> SKSKVDNQFYSVEVGDSTFTVLKRYQNLKPIGSGAQGIVCAAYDAVLDRNVAIKKLSRPFQNQTHAKRAYRELVLMKCVNHKNIISLLNVFTPQKTLEEFQDVYLVMELMDANLCQVIQMELDHERMSYLLYQMLCGIKHLHSAGIIHRDLKPSNIVVKSDCTLKILDFGLARTAGTSFMMTPYVVTRYYRAPEVILGMGYKENVDIWSVGCIMGEMVRHKILFPGRDYIDQWNKVIEQLGTPCPEFMKKLQPTVRNYVENR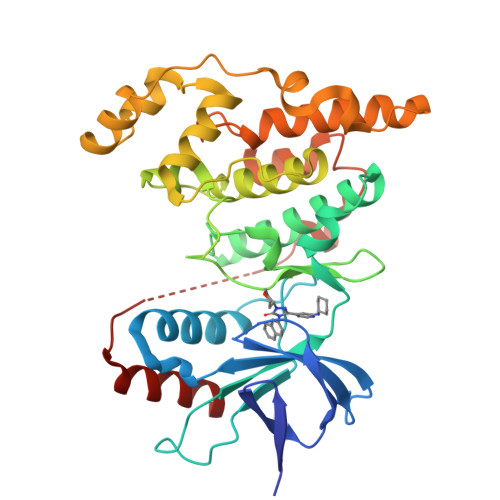PKYAGLTFPKLFPDSLFPADSEHNKLKASQARDLLSKMLVIDPAKRISVDDALQHPYINVWYDPAEVEAPPPQIYDKQLDEREHTIEEWKELIYKEVMNS> SNAKIPNPQPVQLRIPSYGLLKNLTWMPQERRKPKSTEVEVQIKAVPVNFREVLNVLGIFQEYIKKRYRSGIISAENLTFGVEGVGTVVAVGSDVSQWKVGDEVILAYPGNAFSSFVICSPDDLLAKPSDLSMVEAATIFMSFFTAYYGLHNLAKVQPGERVLIHAASGGAGQAAVQLAQFFGSEVFATTSPHKISVLREQGIKHVMNSRTTEFASEVRELTQGNGVDVIFNSLTHGEYIPKNIDILAPGGRYIEIGRLNI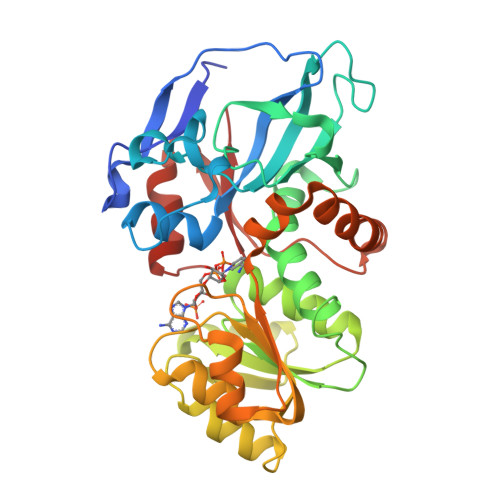WSHEQVSQRRPDVKYFPFDMSDEFVRDKQFHAKLWDDLALLFESGSLKPLPYKVFPSEDVVEAFRHLQHSKHIGKIVVTMP>MAHHHHHHMAEFSIIDQYFNRQSHPDVALGIGDDSALITPPPNQQLVICADTLVAGRHFPLETSPHAIGWKSVAVNLSDIAAMGAKPHSILLAISLPQVDHEWLEGFSQGIYDCCNQFGVALIGGDTTQGPHLTITVTAMGWIETGKAVLRSGAKVGDYVCVSGQIGDAAYGLQHLGHSLQQRLDYPTPRCKLGEELKGLASSMIDVSDGLAQDLGHILKASKVGARLILEKLPVDPVLQQIEEQQRWQYALAGGDDYELCFTITPQNYEKLLQKQLDVKITMIGQIVEQTKLTFEHLGSDYPLQIHGYQHFA[2x]

Thiamine pyrophosphate (TPP) is the biologically active form of vitamin B1 (thiamine) and is essential for all living organisms. The same study also identified genes essential for growth on nutrient agar using high-density transposon mutagenesis, and found thiamine monophosphate kinase (ThiL) to be essential. In this study, we present high-resolution crystal structures of ThiL from the pathogen Acinetobacter baumannii (AbThiL) bound to substrate Thiamine monophosphate (TMP) and substrate analog adenylyl-imidodiphosphate (AMPPNP), and bound to its products TPP and adenosine diphosphate (ADP). The AbThiL structures assume the same two domain fold as MfThiL and AaThiLwith an N-terminal A domain and a C-terminal B domain.

As part of the standard SSGCID pipeline, AbThiL was initially crystallized as apo protein and with AMPPNP/MgCl2. Diffraction was much better for nucleotide-bound protein. Initially, AbThiL was co-crystallized with 5 mM AMPPNP/MgCl2. Crystals from condition JCSG+ G10 (20% w/v PEG 2000MME, 150 mM NaBr) were cryoprotected in two steps with reservoir with 15% v/v ethylene glycol (EG), 5 mM AMPPNP/MgCl2 added, and vitrified by plunging them in liquid nitrogen. A strong anomalous signal for both sites (13.4 and 8.3 sigma) in the AMPPNP-bound structure was additional evidence for potassium, even though no potassium was added during crystallization. By comparison the anomalous density for the phosphorous atoms in AMPPNP is slightly weaker with 7.9 sigma. The anomalous scattering coefficient at CuKα radiation is twice as high for potassium as it is for phosphorous. All of the structures were well resolved: For the structures bound to the substrate/product pairs, residues Met1 or Ala2 through Phe304 or the C-terminal Ala305 could be modeled, while for the AMPPNP-bound structure residues Glu3 through Ile298 were modeled.>MVKETHRFETFTEEPIRLIGEEGEWLGDFPLDLEGEKLRRLYRDMLAARMLDERYTILIRTGKTSFIAPAAGHEAAQVAIAHAIRPGFDWVFPYYRDHGLALALGIPLKELLGQMLATKADPNKGRQMPEHPGSKALNFFTVASPIASHVPPAAGAAISMKLLRTGQVAVCTFGDGATSEGDWYAGINFAAVQGAPAVFIAENNFYAISVDYRHQTHSPTIADKAHAFGIPGYLVDGMDVLASYYVVKEAVERARRGEGPSLVELRVYRYGPHSSADDDSRYRPKEEVAFWRKKDPIPRFRRFLEARGLWNEEWEEDVREEIRAELERGLKEAEEAGPVPPEWMFEDVFAEKPWHLLRQEALLKEEL[2x];>MALMTMVQALNRALDEEMAKDPRVVVLGEDVGKRGGVFLVTEGLLQKYGPDRVMDTPLSEAAIVGAALGMAAHGLRPVAEIQFADYIFPGFDQLVSQVAKLRYRSGGQFTAPLVVRMPSGGGVRGGHHHSQSPEAHFVHTAGLKVVAVSTPYDAKGLLKAAIRDEDPVVFLEPKRLYRSVKEEVPEEDYTLPIGKAALRREGKDLTLICYGTVMPEVLQAAAELAKAGVSAEVLDLRTLMPWDYEAVMNSVAKTGRVVLVSDAPRHASFVSEVAATIAEDLLDMLLAPP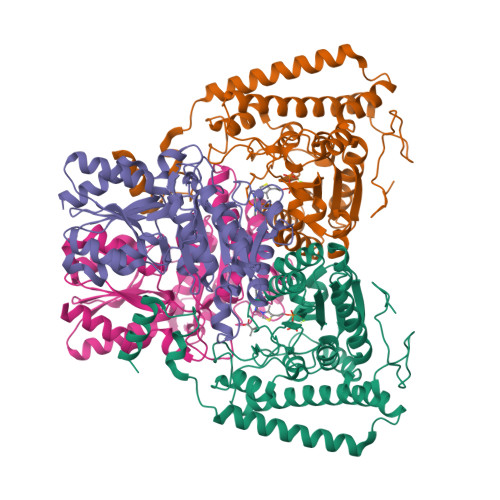IRVTGFDTPYPYAQDKLYLPTVTRILNAAKRALDY[2x]2-oxo-1,2-dihydropyridine-3-carboxylic acid | C6 H5 N O3 | 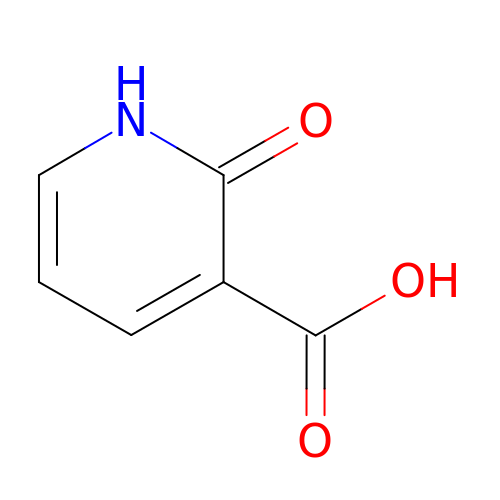UEYQJQVBUVAELZ-UHFFFAOYSA-N> MATSFQFDGLKPSFSASYSSK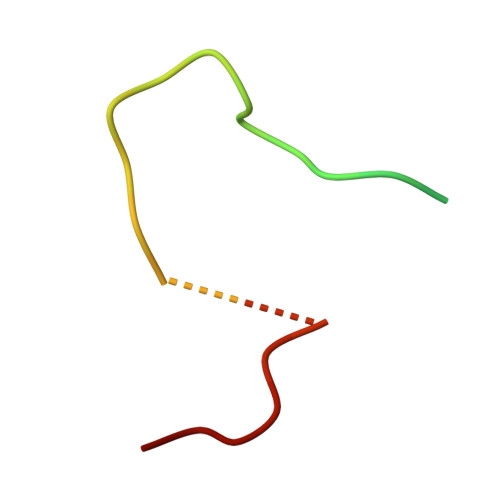PIQTQVSNGMDNASAPV OROTIC ACID | C5 H4 N2 O4 | 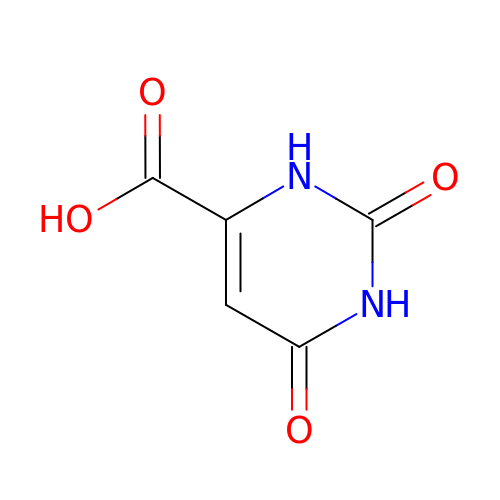PXQPEWDEAKTCGB-UHFFFAOYSA-N> MQKEGVLRVITRNSPATYFQDRNGETGFEYELAKRFAERLGVELKIETADNLDDLYA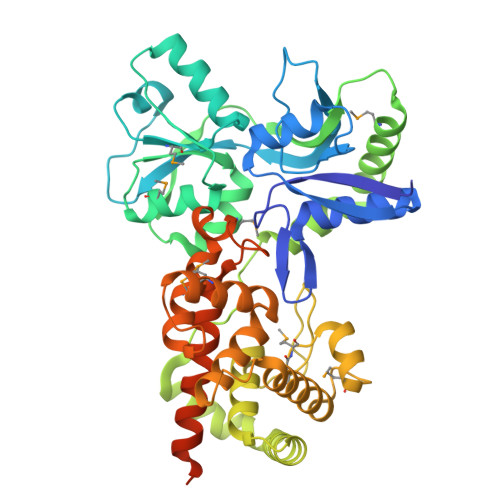QLSREGGPALAAAGLTPGREDDASVRYSHTYLDVTPQIIYRNGQQRPTRPEDLVGKRIMVLKGSSHAEQLAELKKQYPELKYEESDAVEVVDLLRMVDVGDIDLTLVDSNELAMNQVYFPNVRVAFDFGEARGLAWALPGGDDDSLMNEVNAFLDQAKKEGLLQRLKDRYYGHVDVLGYVGAYTFAQHLQQRLPRYESHFKQSGKQKDTDWRLLAAIGYQESLWQPGATSKTGVRGLMMLTNRTAQAMGVSNRLDPKQSIQGGSKYFVQIRSELPESIKEPDRSWFALAAYNIGGAHLEDARKMAEKEGLNPNKWLDVKKMLPRLAQKQWYAKTRYGYARGGETVHFVQNVRRYYDILTWVTQPQMEGSQIAESGLHLPGVNKTRPEEDSGDEKL>MGSSHHHHHHSSGRENLYFQGMATITLERDGLQLVGTREEPFGEIYDMAIIFHGFTANRNTSLLREIANSLRDENIASVRFDFNGHGDSDGKFENMTVLNEIEDANAILNYVKTDPHVRNIYLVGHAQGGVVASMLAGLYPDLIKKVVLLAPAATLKGDALEGNTQGVTYNPDHIPDRLPFKDLTLGGFYLRIAQQLPIYEVSAQFTKPVCLIHGTDDTVVSPNASKKYDQIYQNSTLHLIEGADHCFSDSYQKNAVN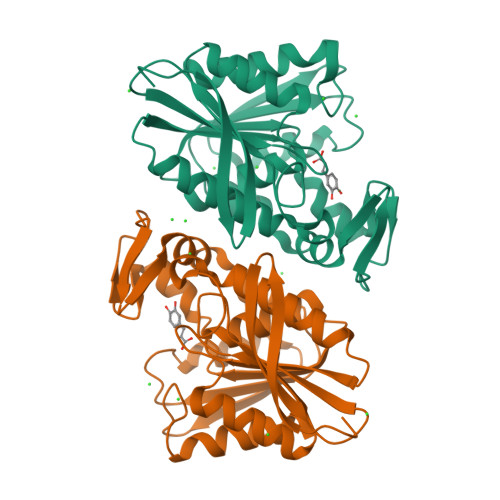LTTDFLQNNNAF[2x]> MPQDPRHPEHQYLDLVKHILENGARRMDRTGTGTLSVFGATMRFSLEDNTFPLLTTRRVFYRGVVEELLFFLRGETDSKVLEKKGVRIWEKNGAKQFLQSVGIDREEGDLGPIYGFQWRHFGARYETSASSYEGKGVDQIASAIAAIRANPASRRIVVSAWNPTDLGSM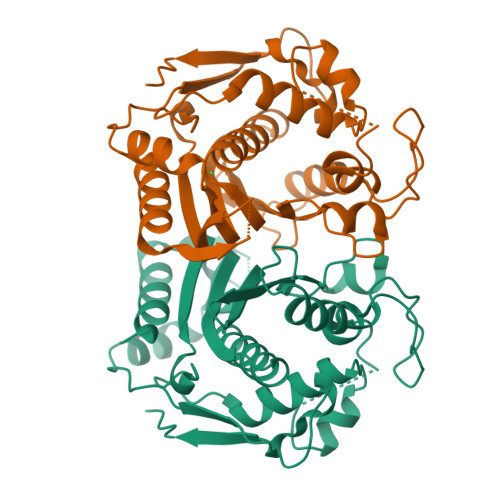ALPPCHVLFQFNVTDGKLSCAMYQRSGDMGLGVPFNIASYSLLTILVAHLTGLQPGEFVHFLGDAHVYLDHVDSLRQQIQRPPRAFPKLFVSPKGPRTEPEHFQYEDFELVGYDPHPAIKMNMSA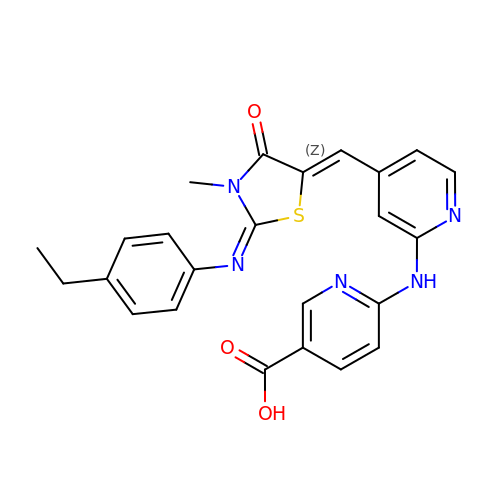6-({4-[(Z)-{(2Z)-2-[(4-ethylphenyl)imino]-3-methyl-4-oxo-1,3-thiazolidin-5-ylidene}methyl]pyridin-2-yl}amino)pyridine-3-carboxylic acid | C24 H21 N5 O3 S | ZJQWORQRPDYKRS-KGQWDEOMSA-N> MWVYRLKGTLEALDPILPGLFDGGARGLWEREGEVWAFFPAPVDLPYEGVWEEVGDEDWLEAWRRDLKPALAPPFVVLAPWHTWEGAEIPLVIEPGMAFGTGHAETTRLALKALARHLRPGDKVLDLGTGSGVLAIAAEKLGGKALGVDIDPMVLPQAEANAKRNGVRPRFLEGSLEAALPFGPFDLLVANLYAELHAALAPRYREALVPGGRALLTGILK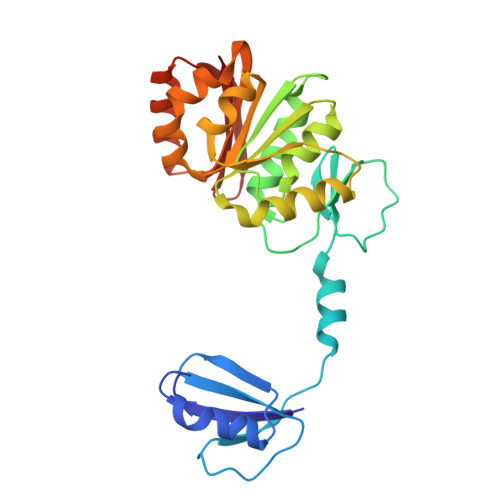DRAPLVREAMAGAGFRPLEEAAEGEWVLLAYGR> APADNTVNIKTFDKVKNAFGDGLSQSAEGTFTFPADVTTVKTIKMFIKNECPNKTCDEWDRYANVYVKNKTTGEWYEIGRFITPYWV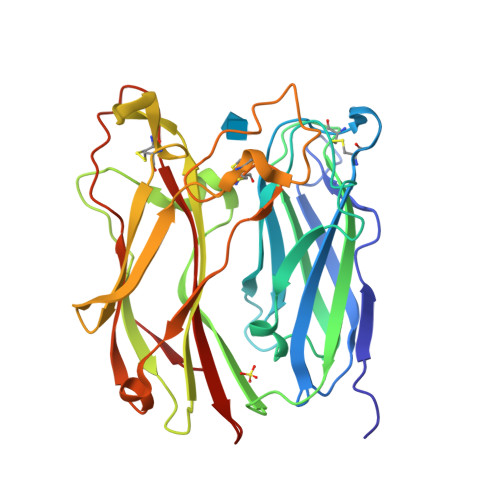GTEKLPRGLEIDVTDFKSLLSGNTELKIYTETWLAKGREYSVDFDIVYGTPDYKYSAVVPVIQYNKSSIDGVPYGKAHTLGLKKNIQLPTNTEKAYLRTTISGWGHAKPYDAGSRGCAEWCFRTHTIAINNANTFQHQLGALGCSANPINNQSPGNWAPDRAGWCPGMAVPTRIDVLNNSLTGSTFSYEYKFQSWTNNGTNGDAFYAISSFVIAKSNTPISAPVVTN> MKVAVLPGDGIGPEVTEAALKVLRALDEAEG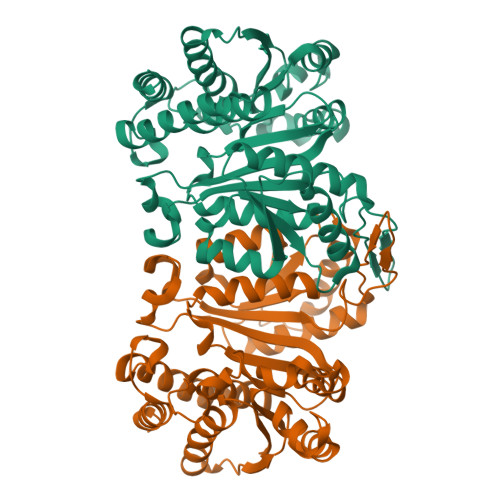LGLAYEVFPFGGAAIDAFGEPFPEPTRKGVEEAEAVLLGSVGGPKWDGLPRKIRPETGLLSLRKSQDLFANLRPAKVFPGLERLSPLKEEIARGVDVLIVRELTGGIYFGEPRGMSEAEAWNTERYSKPEVERVARVAFEGARKRRKHVVSVDKANVLEVGEFWRKTVEEVGRGYPDVALEHQYVDAMAMHLVRSPARFDVVVTGNIFGDILSDLASVLPGSLGLLPSASLGRGTPVFEPVHGSAPDIAGKGIANPTAAILSAAMMLEHAFGLVELARKVEDAVAKALLETPPPDLGGSAGTEAFTATVLRHLA> MGSSHHHHHHSSGKLMSKNIKILVVGAGIAGPAICYWLKRFGFSPVLIEKYASIRKGGQALDIRGIATHLARVMGIYDQICDRRTRIECGRFVDSAGKVLHEEHGEKFGFRQDDEVEILRGDLVEILMKTIADVPCYFNKSIISMQQNADKVIVKFKDGKIENYDIVIGADGIHSATRRMIFDKNEYQLIHLGSYLSTFTIPNYLGLSHTDLECEANHKLVSINSDNNPEIARAGFMFRSQHILKDIRDEHEQKQFLCDTFRDFGWETQNILNRMPESDDFYFDAITQVRMNSWTKGRIALIGDAGYCPSPLSGQGNNLAFVGAYILAGELKTANANYMQAFSRYNALLRSFVDTNQEFGVWVSKSFLVEDEVSKEIAEERSNRILAMIKLVSNAIILPQYE

Tetracycline destructases (TDases) are flavin monooxygenases which can confer resistance to all generations of tetracycline antibiotics. Type 2 TDases have thus far been predominantly identified through soil functional metagenomics with one sequence found in the soil-derived human pathogen Legionella longbeachae. These two types differ in their resistance profiles, with type 1 enzymes conferring resistance to all tetracycline antibiotics including third-generation drugs while type 2 enzymes are generally limited to only first- and second-generation tetracyclines. We determined the X-ray crystal structures of two of these new sequences from Legionella species, and confirmed anhydrotetracycline can inhibit these enzymes’ inactivation of tetracycline antibiotics.

Tet(56-2) and Tet(56-3) are most closely related to Tet(56), at 87.4% and 87.9% amino acid identity respectively, and have 88.6% amino acid identity to each other. Tet(56-2) and Tet(56-3) were also identified in the genomes of Legionella species: L. clemsonensis and L. massiliensis, respectively. We determined the X-ray structures of Tet(56-2) at 1.80 resolution with Rfree/Rwork of 17.43/20.93 and Tet(56-3) at 2.39 Å with Rfree/Rwork of 21.69/24.85. The structures of Tet(56-2) and Tet(56-3) show that the FAD binds in an “OUT” conformation, a conformation that was previously confirmed in X-ray structures of other type 2 TDases. Additionally, we observed that the loop containing F95 shows a distinct conformation in the Tet(56-2) structure, in which F95 is oriented away from the substrate-binding channel, thus presenting the loop with an opening for substrate to enter the active site. The FAD-interacting residues are conserved between both structures. While the apparent catalytic efficiencies (kapp/KM) of Tet(56-2) and Tet(56-3) are similar to Tet(50) for the inactivation of tetracycline and doxycycline, the KM and kapp for the inactivation of doxycycline by Tet(56-2) are 150 ± 42 µM and 3.2 ± 0.2 min−1 respectively. This is much larger than that of Tet(50) (KM and kapp values of 3.57 ± 0.44 μM and 0.15 ± 0.02 min−1 respectively), suggesting that while Tet(56-2) has a much lower binding affinity for doxycycline, the turnover rate is higher. The addition of 1 μg/mL anhydrotetracycline reduced the concentration of tetracycline required to inhibit the growth of Tet(56-2) producing E. coli two-fold, from 32 μg/mL to 16 μg/mL. Apparent IC50 values for anhydrotetracycline inhibition of Tet(56-2) and Tet(56-3) were in the low micromolar range (0.3-30 µM) for tetracycline and doxycycline inhibition.> QKEMDRKGLLGYYFKDKDFSNLTMFSPTRYNTLIYDQQTANKLLDKKQQEYQSIRWIGLIQSNKTGDFTFELSDDECAIIEMDGKVISNKGKEKQVVHLEKGKLVPIKIEYQLDEPLNIDDEKFKGFKLLKVDNQKQLHQVQQDELRNPEFNKKESQEFLAKASKINLFTKKIKRDIDEGTDTDGDSIPDMWEENGYTIQNRIAVKWNDSLASKGYTKFVSNPLDSHTVGDPYTDYEKASRDLDLSNAKETFNPLVAAFPSVNVSMEKVILSPNKNLSNSVESHSSTNWSYTNTEGASVEAGIGPKGFSFGVSANYQHSETVAQEWGASIGDTTQLNTASAGYLNANVRYNNVGTGAIYDVKPTTSFVLEKNTIATITAKSNSTALSISPGESYPKKGQNGIAITSMDDFNSHPITLNKKQLDQVLTNNPIMLETDQTDGIYKIKDTHGNIVTGGTWNGVTQQIKAKTASII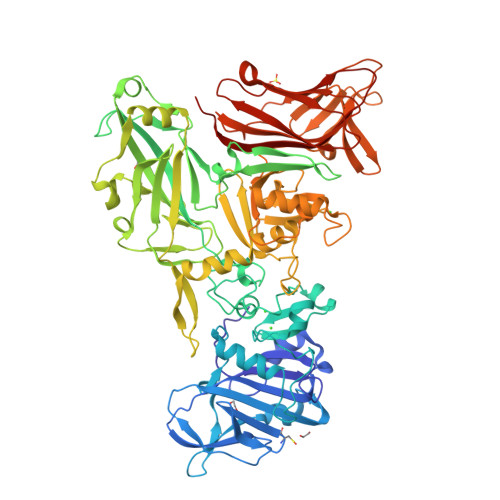VDDGKQVAEKRVAAKDYAYPEDKTPSLTLKDALKLSFPEEIKETDGLLYYNNKPIYESSVMTYLDGNTAKEVKKQINDKTGEFKDVQHLYAVKLTPKMNFTIKVPVAYDTAKQAVNLGGDNPWGAKGLLGTWVNAMVVDNSGDKAYKRVEPGYLLSPTLEFSEGSLDNLKKNYSFYVSMYVKSDKPFTLRINAGPYSTKRTIEASNDFKRVDIPAFYIEGFPIDTIRLEGSDYPSAIWWKDVSITEVSAVKK> MTGGLVLNAISRAGGAMGGLGLIKSLAEKEKQLLERLEAAKKEAEERVKRAEAEAKALLEEAEAKAKALEAQYRERERAETEALLARYRERAEAEAKAVREKAMARLDEAVALV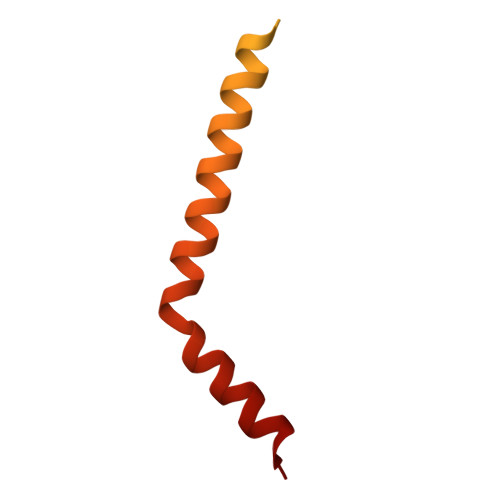LKEVLP>[2x]MGFKQDIATIRGDLRTYAQDIFLAFLNKYPDERRYFKNYVGKSDQELKSMAKFGDHTEKVFNLMMEVADRATDSVPLASDANTLVQMKQHSSLTTGNFEKLFVALVEYMRAS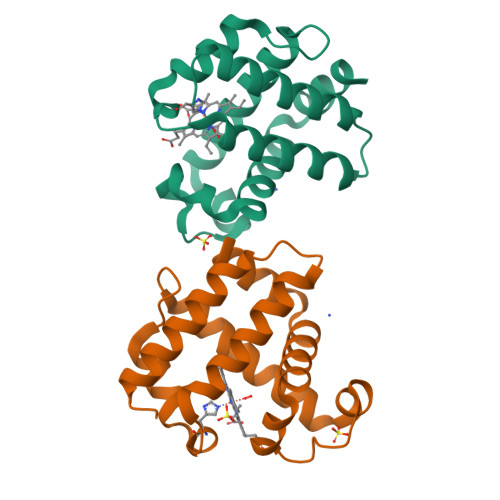GQSFDSQSWDRFGKNLVSALSSAGMK> GDQVEQSPSALSLHEGTDSALRCNFTTTMRSVQWFRQNSRGSLISLFYLASGTKENGRLKSAFDSERARYSTLHIRDAQLEDSGTYFCAAEASSGSWQLIFGSGTQLT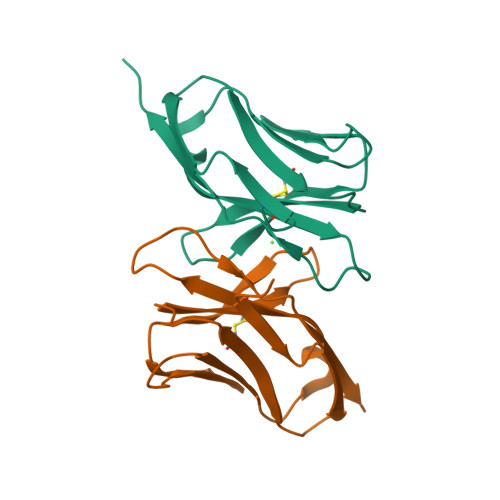VMPVT;>[2x]GDQVEQSPSALSLHEGTDSALRCNFTTTMRSVQWFRQNSRGSLISLFYLASGTKENGRLKSAFDSKERRYSTLHIRDAQLEDSGTYFCAAEASSGAWQLIFGSGTQLTVMPVT;> GDQVEQSPSALSLHEGTDSALRCNFTTTMRSVQWFRQNSRGSLISLFYLASGTKENGRLKSAFDSKERRYSTLHIRDAQLEDSGTYFCAAEASSGSWQLIFGSGTQLTVMPVT>MATRIEFHKHGGPEVLQAVEFTPADPAENEIQVENKAIGINFIDTYIRSGLYPPPSLPSGLGTEAAGIVSKVGSGVKHIKAGDRVVYAQSALGAYSSVHNIIADKAAILPAAISFEQAAASFLKGLTVYYLLRKTYEIKPDEQFLFHAAAGGVGLIACQWAKALGAKLIGTVGTAQKAQSALKAGAWQVINYREEDLVERLKEITGGKKVRVVYDSVGRDTWERSLDCLQRRGLMVSFGNSSGAVTGVNLGILNQKGSLYVTRPSLQGYITTREELTEASNELFSLIASGVIKVDVAEQQKYPLKDAQRAHEILESRATQ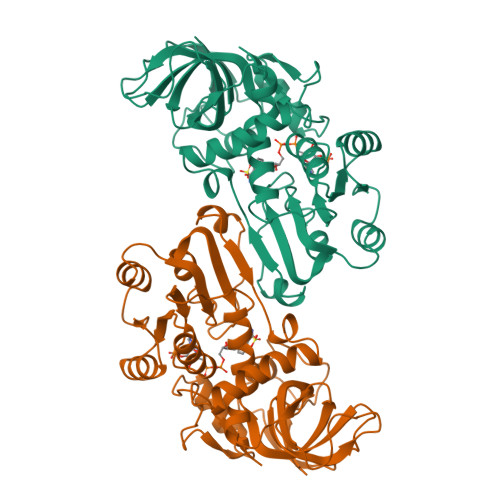GSSLLIP[2x]> MDPYCPFDALDVWEHRRFIVADSRNFITPEFPRDFWMSPVFNLPRETAAEQVVVLQAQRTAAAAALENAAMQAAELPVDIERRLRPIERNVH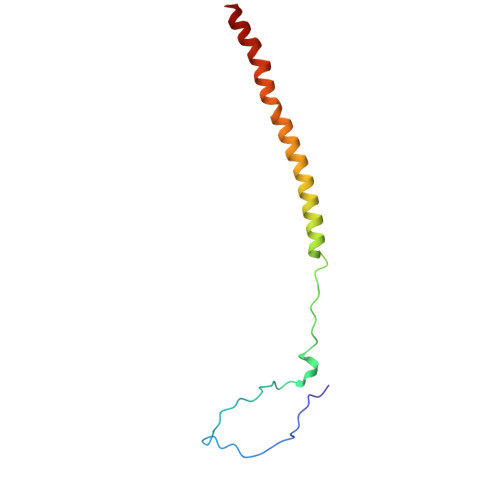EI Insulin binds with high affinity to the insulin receptor (IR), while IGF-1 binds with highest affinity to the IGF-1 receptor (IGF1R)2. For both receptors, ligand binding activates intrinsic receptor tyrosine kinase activity and downstream signalling cascades, which in turn regulate gene transcription, glucose, lipid and protein metabolism as well as cell growth and differentiation. The NPEY motif within the juxtamembrane region of the IR has previously been shown to be critical for the recruitment of receptor substrates, including Shc and IRS-1. By point-mutational and structural modelling, we have identified one amino acid in the juxtamembrane region of the ICD of the two receptors that determines substrate preference and plays a major role in differentiating IR and IGF1R action with respect to both signalling and gene expression.

To explore the structural basis of the substrate preference and the role of the Leu to Phe change at the NPEY+1 position, we compared the previously reported structures of the Shc and IRS-1 phosphotyrosine-binding domains (PTB domains) bound to the phosphorylated NPEY motif peptides. The crystal structure of the IRS-1 PTB domain was determined in complex with a peptide representing the juxtamembrane region of the IR, which has a Leu in the Y+1 position25. Both the Shc and IRS-1 PTB domains bind the receptor peptide in a generally similar manner. The four to five residues immediately N terminal to the NPEY motif form a β-strand that is sandwiched between the C-terminal α-helix and strand β5 of the PTB domain, while the NPEY motif forms a turn that positions the phosphorylated tyrosine in a positively charged pocket. However, unlike the IRS-1 PTB domain, the Shc-PTB domain contains a large insertion that creates a hydrophobic pocket that coordinates the phenylalanine residue in the Y+1 position. In contrast, the crystal structure of IRS-1 PTB domain complexed with a phosphorylated NPEY segment of the IR25 lacks the Y+1 recognition pocket for Phe, while preserving a pY binding pocket and similar cleft for the N-terminal β-strand of the phosphorylated NPEY peptide. These observations provide a structural rationale for preferential binding of Shc to IGF1R. The additional binding interactions with the phenylalanine in the Y+1 position should allow it to outcompete IRS-1, which lacks the Y+1 pocket. Thus, while the Tyr residue in NPEY motif is essential for substrate recruitment, it is the residues surrounding the NPEY motif that dictate the substrate preference, and a key residue in these interactions is the Leu versus Phe at Y+1 position after NPEY motif.

> KEVWQVILKPKGLGQTKNLIGIYRLCLTSKTISFVKLNSEAAAVVLQLMNIRRCGHSENFFFIEVGRSAVTGPGEFWMQVDDSVVAQNMHETILEAMRAMSDAFR;> XLYASSNPAY> APVRSLNCTLRDSQQKSLVMSGPYELKALHLQGQDMEQQVVFSMSFVQGEESNDKIPVALGLKEKNLYLSCVLKDDK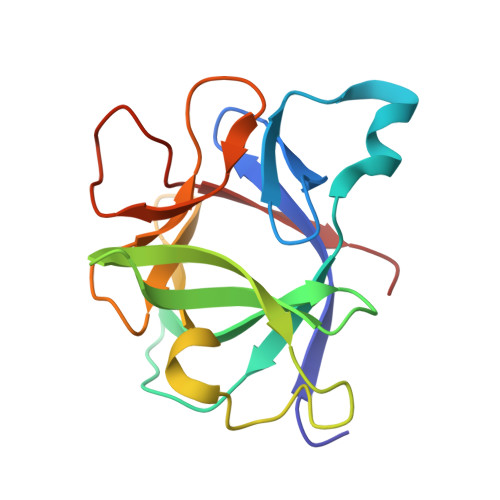PTLQLESVDPKNYPKKKMEKRFVFNKIEINNKLEFESAQFPNWYISTSQAENMPVFLGGTKGGQDITDWTMQFVSS>MQDNSRYTHFLTQHYDAKPQGRDDRYCESIMRRRGLTSPCKDINTFIHGNKRSIKAICENKNGNPHRENLRISKSSFQVTTCKLHGGSPWPPCQYRATAGFRNVVVACENGLPVRLDQSIFRRP[2x]

Angiogenin (ANG), a 14-kDa basic protein is an angiogenic ribonuclease and member of the bovine pancreatic ribonuclease (RNase A) family (also known as RNase 5). Like RNase A, ANG cleaves preferentially on the 3′ side of pyrimidines and follows a transphosphorylation/hydrolysis mechanism. In addition, the crystal structure of human ANG has revealed that it has an RNase A fold and the catalytic triad (residues H13, K40 and H114) is conserved. The enzymatic activity of ANG is several orders of magnitude lower than that of RNase A towards conventional RNase substrates, but essential for its angiogenic effect.

In the H114R ALS variant the protein retains only 2% of the enzymatic activity toward tRNA. H114 is part of the catalytic site (P1) in the native structure and makes direct interaction with D116. However, in the variant structure this interaction is lost and a new van der Waals interaction with L69 has been observed involving the flexible loop region H65-R70. The main chain of R114 also makes an interaction with Q12 (which is known to be part of the substrate-binding site in the native protein). The loss of interaction with D116 also results with movement of C-terminal residues beyond D116 thus causing destablization in the variant structure (where the Arg side chain is more solvent exposed compared with the His residue in the native structure) which will have major impact on the loss of catalytic activity as these residues are implicated in substrate recognition.> MGSWEIDPKDLTFLKELGTGQFGVVKYGKWRGQYDVAIKMIKEGSMSEDEFIEEAKVMMNLSHEKLVQLYGVCTKQRPIFIITEYMANGCLLNYLREMRHRFQTQQLLEMCKDVCEAMEYLESKQFLHRDLAARNCLVNDQGVVKVSDFGLSRYVLDDE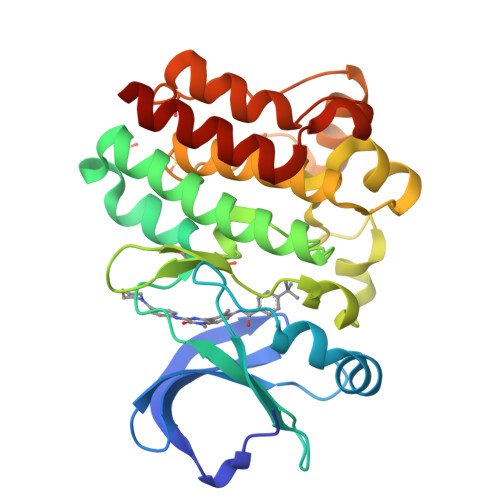YTSSVGSKFPVRWSPPEVLMYSKFSSKSDIWAFGVLMWEIYSLGKMPYERFTNSETAEHIAQGLRLYRPHLASEKVYTIMYSCWHEKADERPTFKILLSNILDVMDENLYGQ>MAPARENVSLFFKLYCLTVMTLVAAAYTVALRYTRTTAEELYFSTTAVCITEVIKLLISVGLLAKETGSLGRFKASLSENVLGSPKELAKLSVPSLVYAVQNNMAFLALSNLDAAVYQVTYQLKIPCTALCTVLMLNRTLSKLQWISVFMLCGGVTLVQWKPAQATKVVVAQNPLLGFGAIAIAVLCSGFAGVYFEKVLKSSDTSLWVRNIQMYLSGIVVTLAGTYLSDGAEIQEKGFFYGYTYYVWFVIFLASVGGLYTSVVVKYTDNIMKGFSAAAAIVLSTIASVLLFGLQITLSFALGALLVCVSIYLYGLPRQDTTSIQQEATSKERIIGVSNSLEVLFQ[2x]

Nucleotide-sugar transporters (NSTs) are products of the solute carrier 35 (SLC35) gene family in humans and are a critical part of the glycosylation machinery in all eukaryotes. They are responsible for transporting nucleotide sugars from the cytoplasm, where they are synthesized, into the Golgi lumen where they are then utilized by glycosyltransferases to glycosylate proteins and lipids. NSTs provide an additional essential role of transporting the nucleotide monophosphate (NMP) byproduct of the glycosyltransferase reaction back to the cytoplasm where it can be recycled. The structure of mCST consists of a 10-TM bundle.

We initially obtained crystals of full-length mCST in complex with CMP using the hanging-drop vapor diffusion (HDVD) method, which diffracted anisotropically to a moderate resolution (3.4 × 3.4 × 4.6 Å). We calculated an experimental electron density map using multiple isomorphous replacement with anomalous scattering using Hg and Pt derivatives. A model based on this map showed that the entire 20-residue C-terminus was disordered. The HDVD and LCP structures were overall very similar, despite having very different crystal lattices. This indicates that the crystal packing interactions had no impact on the overall conformation of mCST. ¶The refinement statistics in this column represent the model from the LCP mCST∆C-CMP crystal being refined against the native HDVD mCST-CMP dataset. We observe several intra-membrane interactions between mCST molecules in our various crystal lattices. However, since we determined that hCST, which is biochemically identical to mCST, is a monomer when purified in detergent, these interactions do not stem from a stable pre-formed oligomer that survived detergent extraction and purification.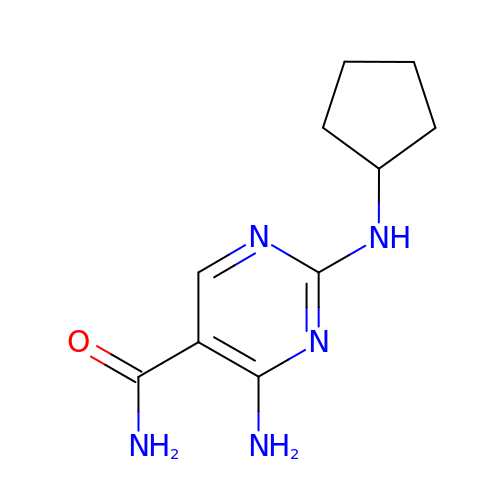4-amino-2-(cyclopentylamino)pyrimidine-5-carboxamide | C10 H15 N5 O | NNNGDGCCKKOXPR-UHFFFAOYSA-N> GSHMEAVQNRIVEA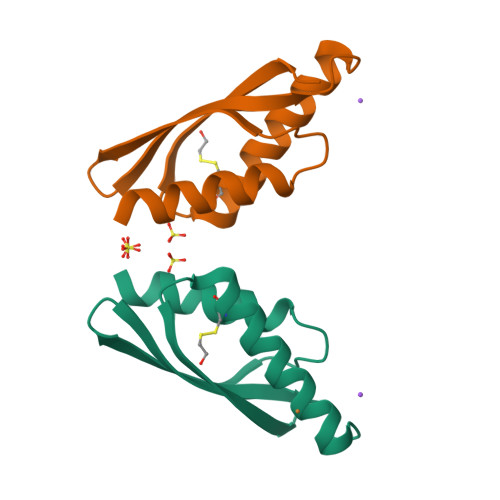AERVPGVRGVIHLRARYVGQDIWAHMIIGVDPENTVEQAHEICEAVQAAVCGKIRRIESLHVSAEAREIGDTTKPSFSDQPLSFDEVMLSKVDN5-O-phosphono-beta-D-arabinofuranose | C5 H11 O8 P | 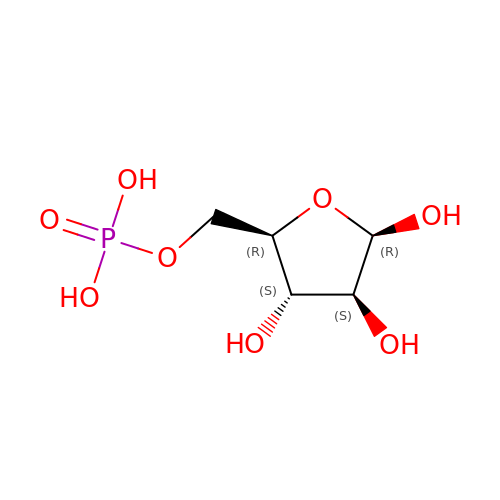KTVPXOYAKDPRHY-SQOUGZDYSA-N>[2x]MTKPLILASQSPRRKELLDLLQLPYSIIVSEVEEKLNRNFSPEENVQWLAKQKAKAVADLHPHAIVIGADTMVCLDGECLGKPQD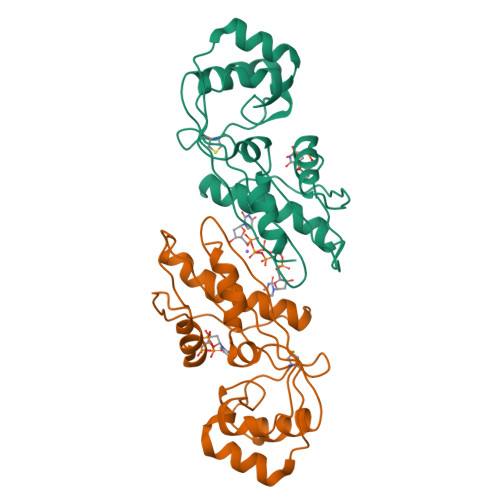QEEAASMLRRLSGRSHSVITAVSIQAENHSETFYDKTEVAFWSLSEEEIWTYIETKEPMDKAGAYGIQGRGALFVKKIDGDYYSVMGLPISKTMRALRHFDIRA>FTLIELMIVVAIIGILAAIAIPQYQNYVA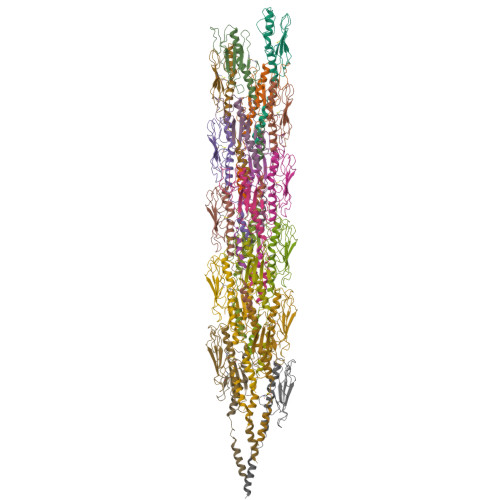RSEGASALASVNPLKTTVEEALSRGWSVKSGTGTEDATKKEVPLGVAADANKLGTIALKPDPADGTADITLTFTMGGAGPKNKGKIITLTRTAADGLWKCTSDQDEQFIPKGCSR[21x]> MDGSRGTAPGGDDLRGDRRDSYQGEDREDSHLLGALEDGNHQQSQGHGGGSGFYHHNVNSSSASVLEGVEMAHDELFAGPVAESVPTSVSAFSHRHGRAESVASFSFYHEQDDQREELEAPPGSLGARLSIDDLDELPFEEEGLSESEMPEQLDTFGIDLEWGSMNNGYPLIRRSSTHSQFSAHHRLLRRESGVSAASGYTGGRSSQKMRLDNDDLTIAISGFITNRIGFAIYIVLCVLTGGIAWLFLRWYPKYYVKLVGCATPFRDCQWVVIEDHFNKMTILSIRVKPYNRPLSTVFGTPSRATSWPLAQDPDPVLRELRSITYCYYKFYYHPVLDKFFCCNGWKDPQWNSMQNARSGLHGDEKAHREAVFGPNSIDVDEQSILQLLVSEILTPFYAFQVFSLILWLCDEYYYYAAAILLISAGSIITSLLETKETRRRLREMSRFECEVRVFRGGFWRTFPSSDLVPGDVYEVSDPSLTQIPADSLLLTGDCIVNESMLTGESVAVSKTPATNETLAKLNPAASTFSHDVDKHFLYCGTKLIRARQRLADTDEAAAVALVVRTGFNTTRGALVRSMLVPKPSKFKFYEDSFRYLKVMGCLAGLAFIVSLVNFIRLKLHWTLILLRALDLLTIVVPPALPATLTIGTSFAVQRLKGKKIFCTSPQRVNVGGKIDLMCFDKTGTLTEEGLDVLGIRVASRVSNRFTELLTNVDDLTWSCDSVSNGDEVKPADHVDGSSLKKDKTKPLDPYRAALYVMASCHSLRIVDGVAVGDPLEVKMFEFTGWSYEEGFIAGEVISTEGRGDISPSIARPPRYMTSQEMSIGEAPPAVGVLRAFDFNPLLRRSSVIARVVGNSGGYALVKGSPECMPEICRPETLPSDFDELLSYYTHAGYRVIACATKRIPKLNLVSVNRMTRDEVESGLDFVGFIIFENKLKPTTTSVIKELLSSNIGTVMITGDNIRTAVSVARQCGIIEEHAHCYMPRFIEGNADDCNAKLRWESINNPALELDPWTLLPMPVPPQTDASLPYDVSNIRNYAIAVTGDVFRWIVDHAPTDVLHRMLVLGKVYARMSPDEKQELVKKFQSIDYSCGFCGDGANDCAALKAADVGISLSEAEASVAAPFTSQIFDIRCVPEVIREGRASLVTSFSCFKYMSLYSFIQFTSVSFLYVSASNLGDFQFLYIDLMLILPIAVFMSWAGPHSKLCAKRPVSDLVSRKVLVPLLSHVFVCVMIQALAWVAVRQQPWYIPPIVDTEKSNIENSENTTLFFASCFEYILSGVVLNAGRPFRQSPLETWPFLSAVAVTLIATLLMLLVPPYWLFEFMQLTWMSWTFKITLIAFGFVYFLIAWTGEHYLFLWLARFLGRMRQRLFKQPKQRKLYKIVKEKLVF

P-type ATPases form a large membrane protein superfamily that couples ATP hydrolysis to the transport of cargo across biological membranes. In human cells, P5B-ATPases execute the active export of physiologically important polyamines such as spermine from lysosomes to the cytosol, a function linked to a palette of disorders. Here we describe a series of cryo-electron microscopy structures of a yeast homolog of human ATP13A2-5, Ypk9, determined at resolutions reaching 3.4 Å, and depicting three separate transport cycle intermediates, including spermine-bound conformations. Ypk9 exhibits ten TM helices and a soluble N-terminal domain (NTD) in close proximity to the membrane, perhaps involved in lipid regulation.

Next, additional structures were determined, all in the presence of SPM, and using N- or C-terminally linked GFP protein. We exploited conditions in the presence again of BeF3− (yielding a structure at 3.7 Å resolution overall, denoted E2P*), or without a similar compound (3.5 Å, E2.PiSPM). Structural analyses to SERCA and ATP11C-CDC50A suggest the SPM-structures are indeed caught in separate E2P and E2.Pi configurations, with the E2.PiSPM structure indicating the presence of cargo is sufficient to stabilize an E2.Pi state. While the E2.Pi structures are highly similar, distinctions are identified between the two recovered E2P states (see further below). However, while we do not detect polyamine indications in the E2Pinhib structure, poor cryo-EM density for SPM, somewhat shifted toward the luminal side compared to the E2.Pi structures are available for E2P*. Based on these observations, we speculate that the affinity for SPM increases from the E2Pinhib to the E2P* and E2.Pi states. The E2P structures exhibit another peculiar feature. Sandwiched in-between the soluble domains, a long continuous density is observed. While poorly resolved in the E2P* data, we assign the stretch to residues D74-G97 of the Ypk9 N-terminus based on visible side chains in the E2Pinhib cryo-EM density. As observed in our E2P* structure, these shifts weaken the interactions between the N-terminal loop and the ATPase core, leading to dissociation of the auto-inhibitory stretch from the soluble A-, P-, and N-domains. Polyamine binding and the coupled dephosphorylation lead to the release of the auto-inhibitory loop, and the formation of a binding pocket between TM 2, 4, and 6 (E2P*).> MSGGGNLLTLERDHFKYLFLTSYFDLKDNEHVPSEPMAFIRNYLNCTFDLLDDAVLMNYFNYLQSMQLKHLVGSTSTNIFKFVKPQFRFVCDRTTVDILEFDTRMYIKPGTPVYATNLFTSNPRKMMAFLYAEFGKVFKNKIFVNINNYGCVLAGSAGFLFDDAYVDWNGVRMCAAPRLDNNMHPFRLYLLGEDMAKHFVDNNILPPHPSNAKTRKINNSMFMLKNFYKGLPLFKSKYTVVNSTKIVTRKPNDIFNEIDKELNGNCPFIKFIQRDYIFDAQFPPDLLDLLNEYMTKSSIMKIITKFVIEENPAMSGEMSREIILDRYSVDNYRKLYIKMEITNQFPVMYD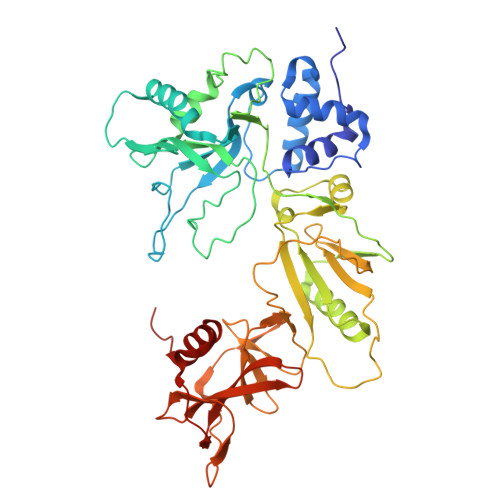HESSYIFVSKDFLQLKGTMNAFYAPKQRILSILAVNRLFGATETIDFHPNLLVYRQSSPPVRLTGDVYVVDKNEKVFLVKHVFSNTVPAYLLIRGDYESSSDLKSLRDLNPWVQNTLLKLLIPDSVQ> AEKQAKRNRREEILQSLALMLESSDGSQRITTAKLAASVGVSEAALYRHF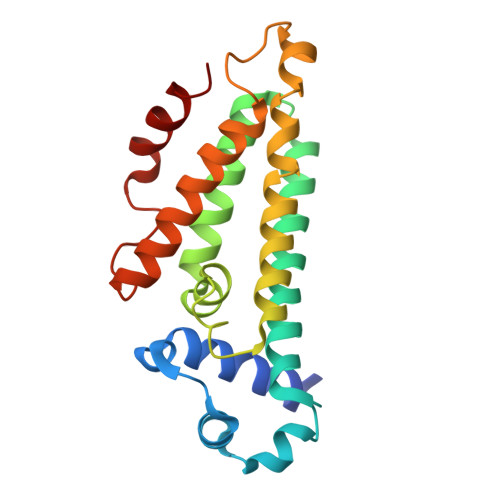PSKTRMFDSLIEFIEDSLITRINLILKDEKDTTARLRLIVLLLLGFGERNPGLTRILTGHALMFEQDRLQGRINQLFERIEAQLRQVLREKRMREGEGYTTDETLLASQILAFCEGMLSRFVRSEFKYRPTDDFDARWPLIAAQLQ> MDNNKAEADTSSSMADPETRPTYTTHHLAIPSGVTQDEFDELKQSVVEFHTYQLSQNQCSSLLAQRIRAPNDVVWSIVRRFDQPQTYKHFIKSCSVSDNFTMAVGSTRDVNVISGLPAATSTERLDILDDDRQVTGFSIIGG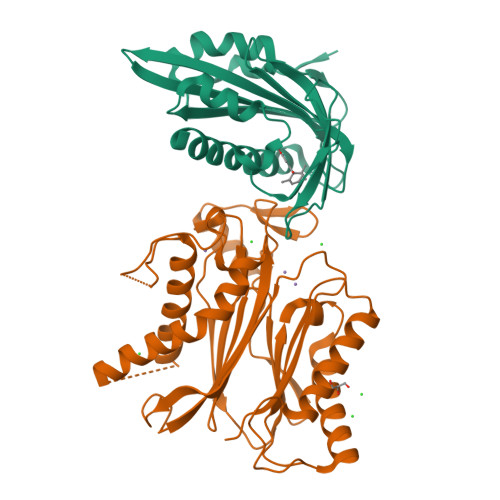EHRLRNYRSVTSVHGFNRDGAICTVVLESYVVDVPEGNTEEDTRLFADTVVKLNLQKLVSVAESQVI;> RSVYELDCIPLWGVVSIQGNRSEMEDAFAVSPHFLKLPIKMLMGDHEGMSPSLTHLTGHFFGVYDGHGGHKVADYCRDRLHFALAEEIERIKDELCKRNTGEGRQVQWDKVFTSCFLTVDGEIEGKIGRAVVGSSDKVLEAVASETVGSTAVVALVCSSHIVVSNCGDSRAVLFRGKEAMPLSVDHKPDREDEYARIENAGGKVIQWQGARVFGVLAMSRSIGDRYLKPYVIPEPEVTFMPRSREDECLILASDGLWDVMNNQEVCEIARRRILMWHKKNGAPPLAERGKGIDPACQAAADYLSMLALQKGSKDNISIIVIDLKAQRKFKTRT>[6x]MLNQELELSLNMAFARAREHRHEFMTVEHLLLALLSNPSAREALEACSVDLVALRQELEAFIEQTTPVLPASEEERDTQPTLSFQRVLQRAVFHVQSSGRNEVTGANVLVAIFSEQESQAAYLLRKHEVSRLDVVNFISHGTRKDEPTQSSDPGSQPNSEEQAGGEERTENFTTNLNQLARVGGIDPLIGREKELERAIQVLCRRRKNNPLLVGESGVGKTAIAEGLAWRIVQGDVPEVMADCTIYSLDIGSLLAGTKYRGDFEKRFKALLKQLEQDTNSILFIDEIHTIIGAGAASGGQVDAANLIKPLLSSGKIRVIGSTTYQEFSNIFEKDRALARRFQKIDITEPSIEETVQIINGLKPKYEAHHDVRYTAKAVRAAVELAVKYINDRHLPDKAIDVIDEAGARARLMPVSKRKKTVNVADIESVVARIARIPEKSVSQSDRDTLKNLGDRLKMLVFGQDKAIEALTEAIKMARAGLGHEHKPVGSFLFAGPTGVGKTEVTVQLSKALGIELLRFDMSEYMERHTVSRLIGAPPGYVGFDQGGLLTDAVIKHPHAVLLLDEIEKAHPDVFNILLQVMDNGTLTDNNGRKADFRNVVLVMTTNAGVRETERKSIGLIHQDNSTDAMEEIKKIFTPEFRNRLDNIIWFDHLSTDVIHQVVDKFIVELQVQLDQKGVSLEVSQEARNWLAEKGYDRAMGARPMARVIQDNLKKPLANELLFGSLVDGGQVTVALDKEKNELTYGFQSAQKHKAEAAH;>[7x]ALVPMVIEQTSRGERSFDIYSRLLKERVIFLTGQVEDHMANLIVAQMLFLEAENPEKDIYLYINSPGGVITAGMSIYDTMQFIKPDVSTICMGQAASMGAFLLTAGAKGKRFCLPNSRVMIHQPLGGYQGQATDIEIHAREILKVKGRMNELMALHTGQSLEQIERDTERDRFLSAPEAVEYGLVDSILTHRNRSHHHHHH;> MGKTNDWLDFDQLAEEKVRDALKPPSMYKVILVNDDYTPMEFVIDVLQKFFSYDVERATQLMLAVHYQGKAICGVFTAEVAETKVAMVNKYARENEHPLLCTLEKA

ClpAP, a two-ring AAA+ protease, degrades N-end-rule proteins bound by the ClpS adaptor. AAA+ proteases, such as ClpAP, consist of a hexameric AAA+ unfoldase (for example, ClpA6) and a self-compartmentalized peptidase (for example, ClpP14). Each ClpA subunit has two AAA+ modules, called D1 and D2, that associate in the hexamer to form two stacked rings. Here we present high-resolution cryo-EM structures of Escherichia coli ClpAPS complexes, showing how ClpA pore loops interact with the ClpS N-terminal extension (NTE), which is normally intrinsically disordered.

Following single-particle cryo-EM analyses, three-dimensional (3D) classification and reconstruction using RELION-3 yielded six density maps (3.22–3.38 Å), representing three general structural classes (I, II and III), with the latter classes being subdivided into IIa/IIb/IIc or IIIa/IIIb subclasses. In two classes, the NTE is bound by a spiral of pore-1 and pore-2 loops in a manner similar to substrate-polypeptide binding by many AAA+ unfoldases. For example, density for the ClpS NTE was present in both the ClpA D1 and D2 rings in classes I and II, but only in the D1 ring of class III. In classes I and II, residues 2–15 of the ClpS NTE were built into density in the D2 portion of the channel, but this NTE region was not visible in class III, presumably as a consequence of its conformational heterogeneity. The register of this ClpS peptide is very similar in each structure, with the C-terminal portion of the NTE (Pro24–Pro25–Ser26) near the top of the ClpA channel, and the N-terminal portion near the bottom of the channel in classes I and II. In classes II and III, the relative height of ClpA subunits was A (highest) > B > C > D > E > F (lowest), whereas in class-I, subunit B was higher than subunit A, resulting in a shallower spiral when aligned to the bottom of the IGL loop and the two flanking ClpP subunits. Previous ClpAP structures and subclasses IIa and IIb show four or five engaged GYVG loops.> SMSKVDVDLGDSLAKVLPTGVKVTIRHISSAPSPCVALFAAPPGEEPESTFCENHFLAVSISPNENEESEVIIFGIEVLVYGTAHLTTIFVSKADSTGYLHLLKNAPKVSLLRLISNAFLSFLVQTHQRPGVRLMVSLFARAQNQYLFPGSIENPEKHVLDDRGLIKWWCRVIDPILREYEPETGSHEKAVDDQTQESAKSSATAFLIVPGCDKFETRGFFPITARSDGKDRPRWLNSYPLHQLCDNPNAPPRCLVPRFPDDPKTRFLIDLDDELPESTGAAGSKENSGHWRSVKSLAQFWEMMSFRQECSAGRLVGFLWLVINPPGLVNSVQMTSSRVASRDVENVLSESAKTTHDATKQKDEAASVSSPPHPSTSGLQTSPIALPGVSSSDTHATVQQ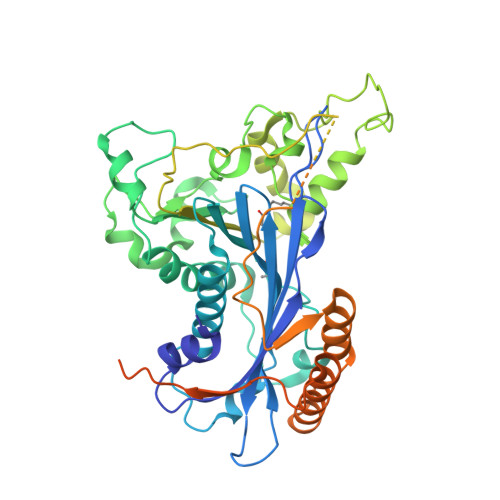ATGPSAFFWPDTGRGHAVLSEEDYKAAINFLIDQDFNTKHKAIASTKAWAEKVASLADQLWVGQRVEGRNATTEPGQKHTDATTVINTAFVRKRKTADEESDKPGEVRGAPGDSEEVNPTPVQSNQAPSVNVLNANLLRKKKKT>GHMSNAAKEVVVVSGVRTAIGDFGGSLKDFSPTDLGAKVVSEVLSRANVSGDAVGHVVFGHVVNTEPKDMYLARVAAINGGVAQHTPALTVNRLCGSGLQAIVSAAQTIMLGDADVAIGGGSENMSRAPYTVPSARFGQRMGDAKLVDMMLGALHDPFQTIHMGVTAENVARKYGITRDAQDALALESHRRAARAIAEGRFKDQILPISIRTKKGEVAFDTDEHVRHDAGPDDFTKLKPVFVKEDGTVTAGNASGINDAAAAVLMM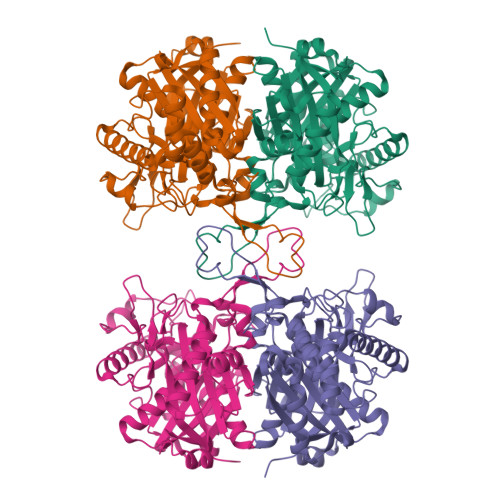SADAARAQGVKPLARLVAYAHAGVDPAYMGIGPVPATQKALERAGLKITDLDVIEANEAFAAQACAVTQELGLDPAKVNPNGSGISLGHPIGATGALITVKALYELKRIGGRYALVTMCIGGGQGIAAIFENI[2x]>MTSAEIRAAFLEFFRQRGHAVRPSSSLVPGNDPTLLFTNAGMVQFKDVFLGREKVDFNRAATSQRCVRAGGKHNDLENVGYTARHHTFFEMLGNFSFGDYFKRDAINFAWDFLTKEMGIPPAKLWVTVFDEDSEAEAIWLEEVKIDPTRFSRIGAKDNFWAMGDVGPCGPCTEIFYDHGEHVAGGPPGSPDEDGDRYIEIWNLVFMQYERDKDGNLTPLPAPSVDTGMGLERIAAVMQGVHSNYEIDIFQNLVKTAAALAGTTDLSNSSLRVIADHIRSCAFLVADGVLPSNEGRGYVLRRIVRRAIRHGYRLGIQDTFFYKLVAPLAAEMGAAYPELVKAQEQVERVLKKEEERFAETLGQGMKILENCVAKLDGHVIPGDVVFLLYDTYGFPVDLTADFAREHNLSVDHAGFEVEMSAQRDRARAGGHHHHHH[2x]

Aminoacyl-tRNA synthetases (AARSs) play a crucial role in the translation of genetic information by attaching specific amino acids to their corresponding transfer RNA (tRNA) molecules. Alanyl-tRNA synthetase (AlaRS) often misactivates Gly or Ser instead of its cognate amino acid, Ala. To get structural explanation why the L219M mutation prevents AlaRS from misactivating Ser to produce seryl-adenylate, we determined the crystal structures of both the wild-type and L219M mutant AlaRS proteins in complex with ATP and Ala. AlaRS429 and AlaRS429L219M consist of the N-terminal nine-stranded β-sheet structure harboring the catalytic site (residues 1–241) and the C-terminal α-helix bundle (residues 242–429) responsible for tRNA recognition.

The N-terminal fragment of AlaRS corresponding to residues 1–429 was used for successful crystallization. Their structures are referred to as AlaRS429 for the wild type and AlaRS429L219M for the L219M mutant. According to the superposed structures of AlaRS429 and AlaRS429L219M, the side chains of Leu219 and Met219 are situated in a hole formed by Pro167, Met206, Glu209, Pro220, Ala221, Pro222, and Ser223 (in motif 3). The only structural difference in the hole between AlaRS429 and AlaRS429L219M is the rotamer change of Glu209, which is since methionine has a linear side chain, but leucine has a branched side chain. However, there is no difference in the position of Val204 observed in the crystal structures of both AlaRS429 and AlaRS429L219M. Leu219 in AlaRS429 and Met219 in AlaRS429L219M contact with the C-terminal segment (residues 206–209) of the β7 strand harboring Val204, and thus the amino acid identity at position 219 could affect the dynamic motion of Val204. Interestingly, the B-values of Cα atoms of Val204 in AlaRS429 and AlaRS429L219M are 19.96 and 26.68 Å2, respectively, suggesting that Val204 is more flexible in AlaRS429L219M than in AlaRS429. That is, the more dynamic Val204 of AlaRS429L219M invades the space intended for the extra hydroxyl group of Ser, whereas the relatively static Val204 in AlaRS429 allows the binding of Ser without inducing clash with the hydroxyl group. Unlike the previous study determining the structures of the post-activation states, our structural studies about both AlaRS429 and AlaRS429L219M in complex with Ala and ATP depicted, for the first time, a visualization of the spatial arrangement of both substrates prior to the activation reaction.> LSECKTGNGKNYRGTMSKTKNGITCQKWSSTSPHRPRFSPATHPSEGLEENYCRNPDNDPQGPWCYTTDPEKRYDYCDILECEEECMHCSGENYDGKI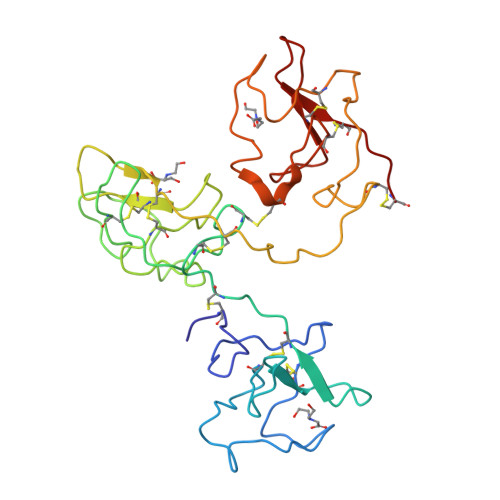SKTMSGLECQAWDSQSPHAHGYIPSKFPNKNLKKNYCRNPDRELRPWCFTTDPNKRWELCDIPRCTTPPPSSGPTYQCLKGTGENYRGNVAVTVSGHTCQHWSAQTPHTHERTPENFPCKNLDENYCRNPDGKRAPWCHTTNSQVRWEYCKIPSC>MAPALNANPTTKRDELSAPSASHKLGMSSMASRAAGGGLKLTGLPDL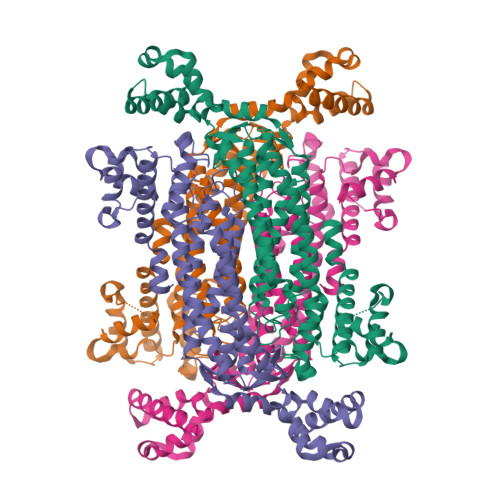SDSAGTLSDIFGTPQMREIWSDQNRVACYLEIEAALAIVQADLGIIPKNAAHEIVEHCRVQEIDWALYKQKTELIIYPVLGIVQQLVANCKDGLGEYCHWGATTQDITDTATVMQIRQSLTLVKQRLDSIVSSLEHLAEQHRNVPMAARSNLKQAVPITFGFKMARFLATFRRHQQRLVELEKRVYTLEFGGAAGNLSSLGDQGIATHDALAKMLDLAPAEIAWHTEHDRFAEVGTFLGLLTGTLAKLATDIKLMSQTEVGEVGEPFISNRGSSSTMPQKNNPISCVYIHACAANVRQGAAALLDAMQSDHEAGTGPWEIIWVQLPLMMNWTSAALNNADFVLRGLQVFPDAMQHNLDLSKGLIVSEAVMMGLGNTLGRQYAHDAVYECCRTAFVQDRPLLDVLLENHEIASKLDRTELEKLCDPANYLGQCSQWIDRVLSPPSSA[4x]> SNRAVAVLRGETVTGTIWITQKSENDQAVIEGEIKGLTPGLHGFHVHQYGDSTNGCISAGPHFNPFGKTH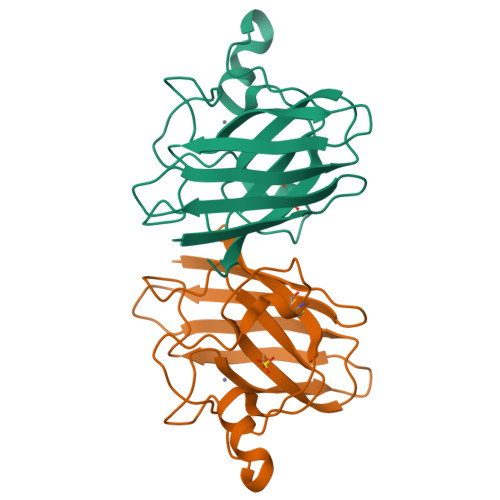GGPKSEIRHVGDLGNVEAGADGVAKIKLTDTLVTLYGPNTVVGRSMVVHAGQDDLGEGVGDKAEESKKTGNAGARAACGVIALAAPQ> STNLKDVLASLIPKEQARIKTFRQQHGNTAVGQITVDMSYGGMRGMKGLIYETSVLDPDEGIRFRGFSIPECQKLLPKAGGGEEPLPEGLFWLLVTGQIPTPEQVSWVSKEWAKRAALPSHVVTMLDNFPTNLHPMSQLSAAITALNSESNFARAYAEGINRTKYWEFVYEDAMDLIAKLPCVAAKIYRNLYRAGSSIGAIDSKLDWSHNFTNMLGYTDPQFTELMRLYLTIHSDHEGGNVSAHTSHLVGSALSDPYLSFAAAMNGLAGPLHGLANQEVLLWLSQLQKDLGADASDEKLRDYIWNTLNSGRVVPGYGHAVLRKTDPRYTCQREFALKHLPSDPMFKLVAQLYKIVPNVLLEQGKAKNPWPNVDAHSGVLLQYYGMTEMNYYTVLFGVSRALGVLAQLIWSRALGF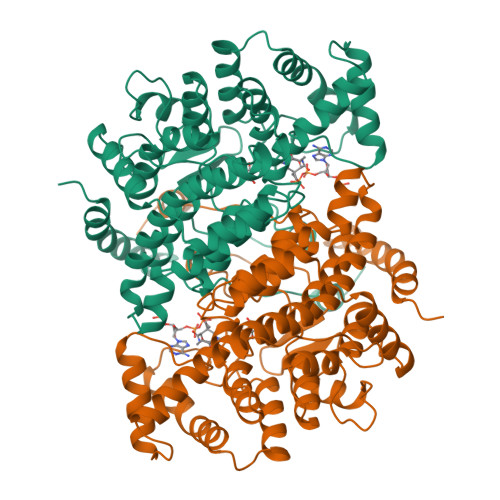PLERPKSMSTAGLEKLSAGG>[2x]QCDVPPNSRFDCAPDKAITQEQCEARGCCYIPAKQGLQGAQMGQPWCFFPPSYPSYKLENLSSSEMGYTATLTRTTPTFFPKDILTLRLDVMMETENRLHFTIKDPANRRYEVPLETPRVHSRAPSPLYSVEFSEEPFGVIVHRQLDGRVLLNTTVAPLFFADQFLQLSTSLPSQYITGLAEHLSPLMLSTSWTRITLWNRDLAPTPGANLYGSHPFYLALEDGGSAHGVFLLNSNAMDVVLQPSPALSWRSTGGILDVYIFLGPEPKSVVQQYLDVVGYPFM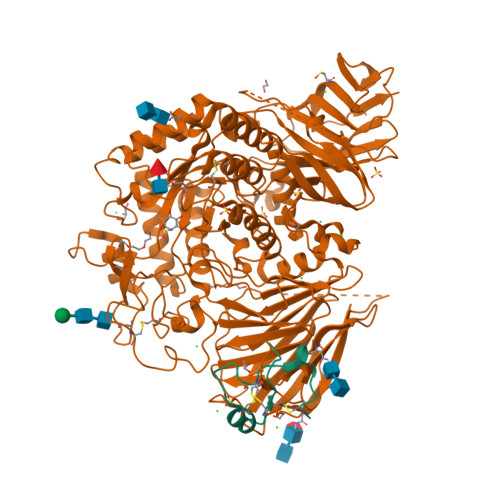PPYWGLGFHLCRWGYSSTAITRQVVENMTRAHFPLDVQWNDLDYMDSRRDFTFNKDGFRDFPAMVQELHQGGRRYMMIVDPAISSSGPAGSYRPYDEGLRRGVFITNETGQPLIGKVWPGSTAFPDFTNPTALAWWEDMVAEFHDQVPFDGMWIDMNEPSNFIRGSEDGCPNNELENPPYVPGVVGGTLQAATICASSHQFLSTHYNLHNLYGLTEAIASHRALVKARGTRPFVISRSTFAGHGRYAGHWTGDVWSSWEQLASSVPEILQFNLLGVPLVGADVCGFLGNTSEELCVRWTQLGAFYPFMRNHNSLLSLPQEPYSFSEPAQQAMRKALTLRYALLPHLYTLFHQAHVAGETVARPLFLEFPKDSSTWTVDHQLLWGEALLITPVLQAGKAEVTGYFPLGTWYDLQTVPIEALGSLPPPPAAPREPAIHSEGQWVTLPAPLDTINVHLRAGYIIPLQGPGLTTTESRQQPMALAVALTKGGEARGELFWDDGESLEVLERGAYTQVIFLARNNTIVNELVRVTSEGAGLQLQKVTVLGVATAPQQVLSNGVPVSNFTYSPDTKVLDICVSLLMGEQFLVSWC>SWCLSVHQPWASLLVRGIKRVEGRSWYTPHRGRLWIAATAKKPSPQEVSELQATYRLLRGKDVEFPNDYPSGCLLGCVDLIDCLSQ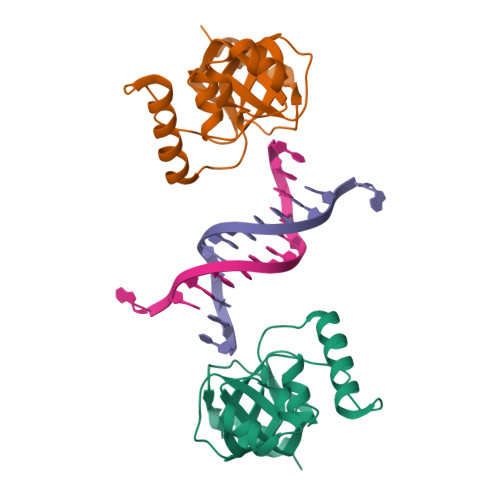KQFKEQFPDISQESDSPFVFICKNPQEMVVKFPIKGNPKIWKLDSKIHQGAKKGLM[2x]>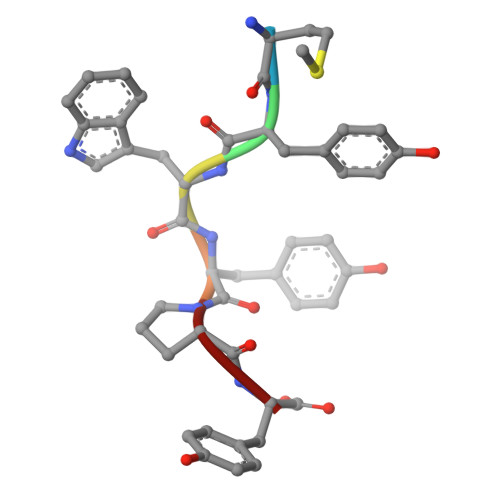 MYWYPY NRZ is a 19 kDa protein expressed in the epiboly of the extra-maternal yolk syncytial layer (YSL) of zebrafish eggs. In vivo, NRZ has been shown to be a potent inhibitor of apoptosis after serum withdrawal, and controls development during somatogenesis and gastrulation. Similar to other pro-survival Bcl-2 proteins, NRZ adopts a conserved Bcl-2-like fold consisting of eight α-helices that form a globular helical bundle. Our findings suggest that NRZ is a unique pro-survival Bcl-2 protein with an unusual pro-apoptotic Bcl-2 binding profile unlike its counterparts in mammalian systems.

To determine the structural basis of NRZ interaction with BH3 motifs of pro-apoptotic Bcl-2 proteins, we determined the crystal structures of apo-NRZ and its complexed holo form bound to the BH3-motif of zBad. Helices α2-5 form the canonical hydrophobic ligand binding groove observed in other Bcl-2 family proteins that is utilized to accommodate the zBad BH3 peptide. Surprisingly, our structural search and comparison using DALI48 revealed that the closest structural homolog of NRZ is in fact Mcl-155 with an R.M.S.D value of 1.7 Å over 136 Cα atoms, and a sequence identity of 15%. In summary, like other pro-survival Bcl-2 protein structures solved to-date, NRZ adopts a Bcl-2 like fold and its most closely related structural homologs are the cellular apoptosis inhibitor Mcl-1 and the canarypox viral Bcl-2 protein CNP058. Comparison of the backbone structures of NRZ and NRZ: zBad BH3 complex. a Cartoon representation of apo NRZ (light blue) superimposed onto NRZ: zBad BH3 complex (green). Here we examined the structure and interactions of NRZ by determining the structures of apo-NRZ and its complex with zBad BH3, the orthologue of mammalian Bad and measuring the binding affinities for BH3-motifs. The structures revealed the conformational changes in NRZ after binding of BH3 motif ligand and provide a structural basis for NRZ mediated apoptosis inhibition.

> GPLSMSCWLREQTLLLAEDYISFCSGIQQTPPSESAEAMRYLAKEMEQQHRTKFRSLSQEFLDTCGADPSKCLQSVMRELVGDGKMNWGRVVSIFTFTGVLASELLSRGENSEGSRRLAETIADYLGGEKQDWLVENGGWEGFCRFFHNARQ> SPNVEACGYSDRVLQLTIGNSTITTQEAANSVVAYGRWPEFIRDDEANPVDQPT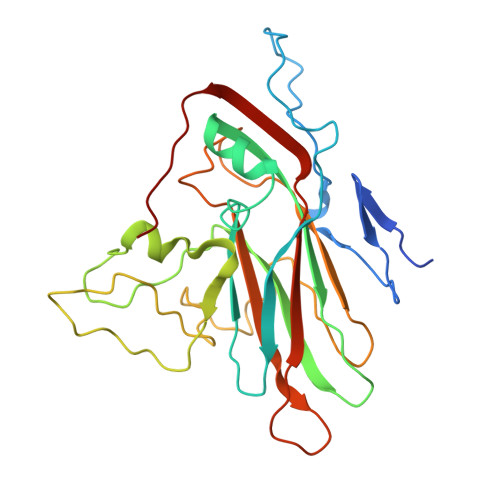EPDVATCRFYTLDTVMWGKESKGWWWKLPDALRDMGLFGQNMYYHYLGRSGYTVHVQCNASKFHQGALGVFAIPEYCLAGDSDKQRYTSYANANPGEKGGKFYSQFNRDTAVTSPKREFCPVDYLLGCGVLLGNAFVYPHQIINLRTNNSATIVLPYVNAMAIDSMVKHNNWGIAILPLSPLDFAQESSVEIPITVTIAPMCSEFNGLRNVTAPKFQ>MKAEIKNLIDRGTYRKLPLFEGELPEGSYAQIVEVKPKQTVKKHYHERQYELFYIISGEARLGIGDTEYQAKPGDIFLVKPKTVHWVVNEKDEPFRLFVVKLNYHGDDSVWLEGSF[4x];> AEIKNLIDRGTYRKLPLFEGELPEGSYAQIVEVKPKQTVKKHYHERQYELFYIISGEARLGIGDTEYQAKPGDIFLVKPKTVHWVVNEKDEPFRLFVVKLNYHG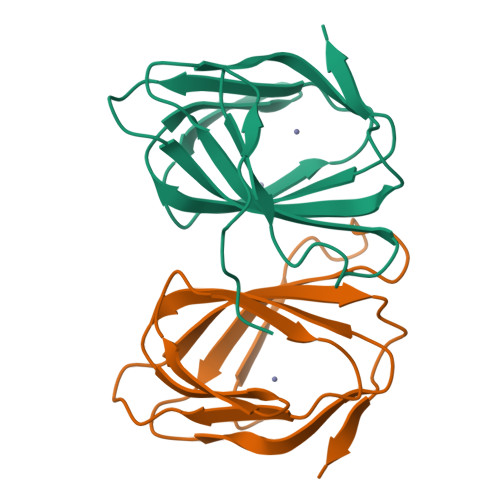DDSVWLEGSF;>[2x]NLIDRGTYRKLPLFEGELPEGSYAQIVEVKPKQTVKKHYHERQYELFYIISGEARLGIGDTEYQAKPGDIFLVKPKTVHWVVNEKDEPFRLFVVKLNYHGDDSVWLEGSF;> GTYRKLPLFEGELPEGSYAQIVEVKPKQTVKKHYHERQYELFYIISGEARLGIGDTEYQAKPGDIFLVKPKTVHWVVNEKDEPFRLFVVKLNYHGDDSVWLEGSF While some archaea produce only one type of filament, the archaeal model species Sulfolobus acidocaldarius generates four. These include rotary swimming propellers analogous to bacterial flagella (archaella), pili for twitching motility (Aap), adhesive fibres (threads), and filaments facilitating homologous recombination upon UV stress (UV pili). Here, we use cryo-electron microscopy to describe the structure of the S. acidocaldarius archaellum at 2.0 Å resolution, and update the structures of the thread and the Aap pilus at 2.7 Å and 2.6 Å resolution, respectively. We define distinct N-glycan patterns in the three filaments and identify a putative O-glycosylation site in the thread.

To facilitate this analyis, we improved the resolution of the structures of the thread and Aap from the previously published resolutions of 3.5 Å15 and 3.2 Å9, to 2.7 Å and 2.6 Å, respectively. Our new cryoEM maps of the archaellum, Aap and thread enabled us to build their complex N-glycans with greater precision. This was particularly the case for the Aap, where N-glycans were previously only partially resolved. Measuring 110 Å, the archaellum is considerably wider than the Aap (80 Å), which is mostly due to the larger head domain of the archaellin. Interestingly, the S. acidocaldarius Aap show an unusual 3-conformer architecture, where each 3-start strand has a distinct conformation. Considering that Aap drive twitching motility in S. acidocaldarius (and likely also in other Sulfolobales species), it is conceivable that the 3-conformer structures are linked to this function, for example enabling rapid retraction. While the Aap has the striking capability to bend up to 90°9, archaella form stable supercoils necessary for swimming motion. On the other hand, Aap do not exhibit the screw-like profile that is caused by the glycosylation domain in the archaellum. In contrast, the diameters of the Aap and archaellum exceed that of either pore, meaning that a local reorganisation of the S-layer would have to take place to accommodate these filaments. With a diameter of 80 Å, Aap would either require a similar local disassembly of SlaA subunits, or at least a significant conformational change of the six SlaA N-termini delineating a hexagonal pore. The Aap’s 3-conformer organisation possibly represents a metastable state that could facilitate the retraction of the filament.

>LSGAIVALILVIAGVIIAIAVVLFAFGLIPGISNQGSIQVLGSGTITNSTASGSSRTIYNITITVKNTGTTSISVTSININGQPFNINGTAPSIPAGRTQPITFEVTPASGKPNFSPGASYTATIYFSNGQGAPATLIYQG[37x]> MSSTPSNQNIIPIIKKESIVSLFEKGIRQDGRKLTDYRPLSITLDYAKKADGSALVKLGTTMVLAGTKLEIDKPYEDTPNQGNLIVNVELLPLAYETFEPGPPDENAIELARVVDRSLRDSKALDLTKLVIEPGKSVWTVWLDVYVLDYGGNVLDACTLASVAALYNTKVYKVEQHSNG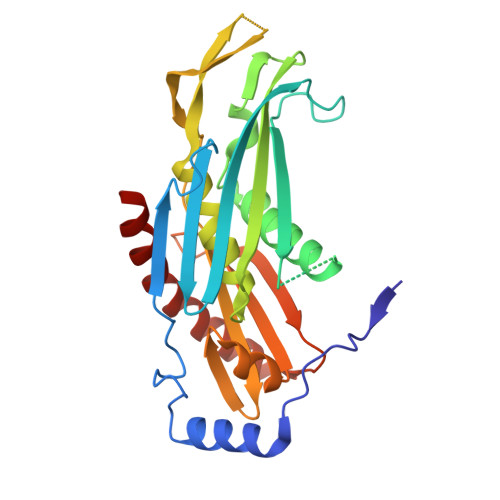ISVNKNEVVGKLPLNYPVVTISVAKVDKYLVVDPDLDEESIMDAKISFSYTPDLKIVGIQKSGKGSMSLQDIDQAENTARSTAVKLLEELKKHLGI>[2x]MALGSLLALLALLLLWGAVAEGPAKKVLTLEGDLVLGGLFPVHQK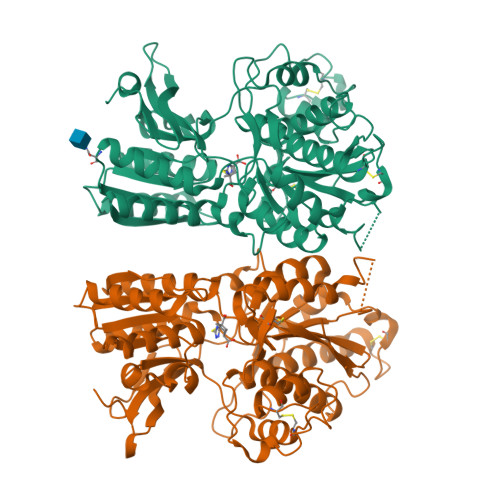GGPAEDCGPVNEHRGIQRLEAMLFALDRINRDPHLLPGVRLGAHILDSCSKDTHALEQALDFVRASLSRGADGSRHICPDGSYATHGDAPTAITGVIGGSYSDVSIQVANLLRLFQIPQISYASTSAKLSDKSRYDYFARTVPPDFFQAKAMAEILRFFNWTYVSTVASEGDYGETGIEAFELEARARNISVATSEKVGRAMSRAAFEGVVRALLQKPSARVAVLFTRSEDARELLAASQRLNASFTWVASDGWGALESVVAGSEGAAEGAITIELASYPISDFASYFQSLDPWNNSRNPWFREFWEQRFRCSFRQRDCAAHSLRAVPFEQESKIMFVVNAVYAMAHALHNMHRALCPNTTRLCDAMRPVNGRRLYKDFVLNVKFDAPFRPADTHNEVRFDRFGDGIGRYNIFTYLRAGSGRYRYQKVGYWAEGLTLDTSLIPWASPSAGEGHHHHHH2-[8-(1,3-benzothiazol-2-ylcarbamoyl)-3,4-dihydroisoquinolin-2(1H)-yl]-5-(3-{4-[3-(dimethylamino)prop-1-yn-1-yl]-2-fluorophenoxy}propyl)-1,3-thiazole-4-carboxylic acid | C35 H32 F N5 O4 S2 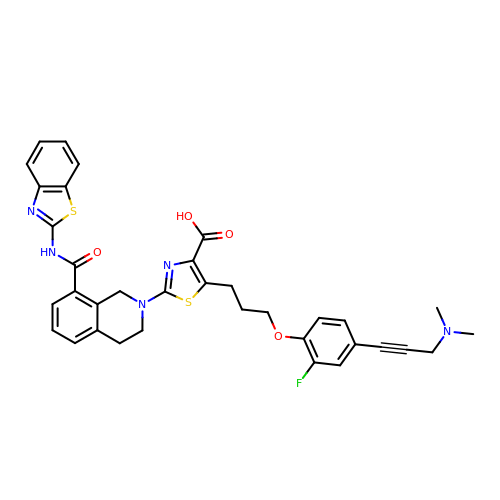| SOYCFODXNRVBTI-UHFFFAOYSA-N> MTQSQTVTVDQQEILNRANEVEAPMADPPTDVPITPCELTAAKNAAQQLVLSADNMREYLAAGAKERQRLATSLRNAAKAYGEVDEEAATALDNDGEGTVQAESAGAVGGDSSAELTDTPRVATAGEPNFMDLKEAARKLETGDQGASLAHFADGWNTFNLTLQGDVKRFRGFDNWEG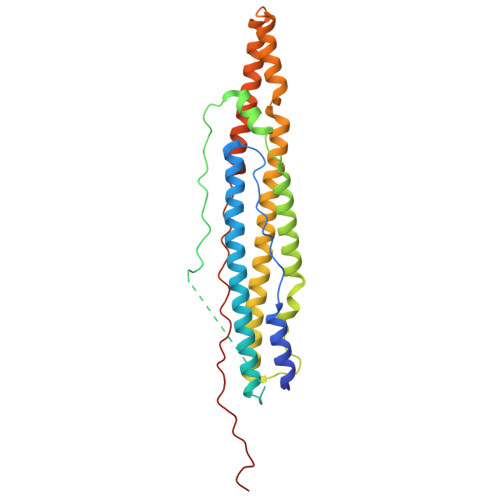DAATACEASLDQQRQWILHMAKLSAAMAKQAQYVAQLHVWARREHPTYEDIVGLERLYAENPSARDQILPVYAEYQQRSEKVLTEYNNKAALEPVNPPKPPPAIKIDPPPPPQEQGLIPGFL> AGIQNDSTGKCGPPPPIDN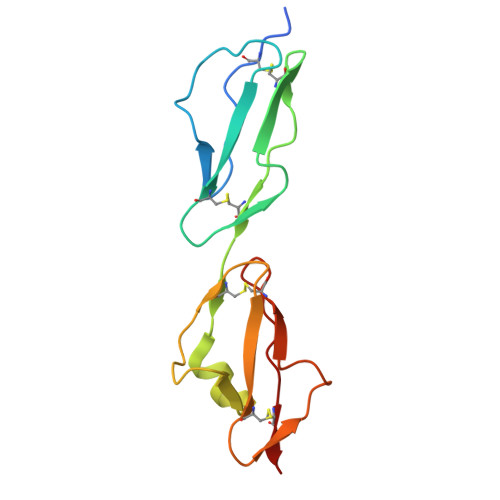GDITSFPLSVYAPASSVEYQCQNLYQLEGNKRITCRNGQWSEPPKCLHPCVISREIMENYNIALRWTAKQKLYSRTGESVEFVCKRGYRLSSRSHTLRTTCWDGKLEYPTCAKR>FDLHTLNWDLCLTQANHKSNLALEMLKMLLDSLPETVEKIQTALGQNDQATMLSTIHKLHGASCYCGVPTTQRLCQEIESALKRQTPVEDLEPEILELLDELTKVESAV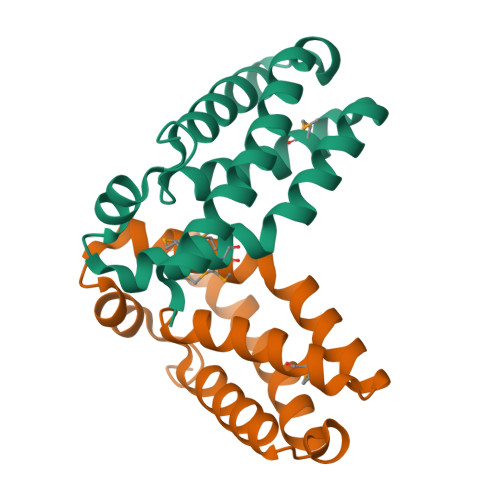KQVLSQLSAE[4x]> GSMALPKDAIPSLSECQCGI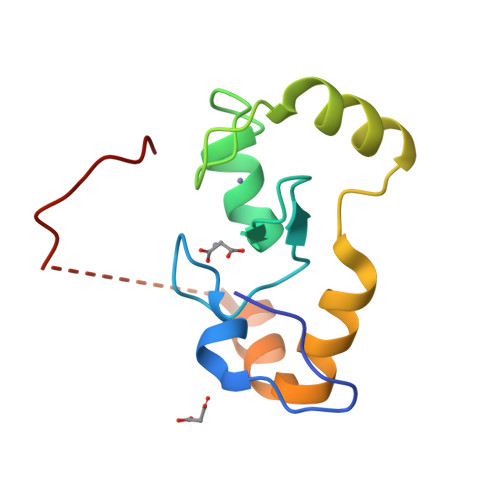CMEILVEPVTLPCNHTLCKPCFQSTVEKASLCCPFCRRRVSSWTRYHTRRNSLVNVELWTIIQKHYPRECKLRASGQESEEVADDYQPVRLLSKP The basic helix-loop-helix PER-ARNT-SIM (bHLH-PAS) domain-containing transcription factor CLOCK:BMAL1 forms the positive component of the core feedback loop. PER and CRY proteins interact with each other to form a large complex with the kinase CK1δ and enter the nucleus after a delay to bind directly to CLOCK:BMAL1 and inhibit its activity. What structural features of CRY1 and CRY2 might lead to differential functions in the circadian clock? Both cryptochromes are defined by a highly conserved photolyase homology region (PHR) domain and divergent C-terminal tails that are intrinsically disordered. However, repression also relies on the recruitment of CRY1 to the PAS domain core of CLOCK:BMAL1 via the CLOCK PAS-B domain, which docks into the evolutionarily conserved secondary pocket on the CRY1 PHR domain.

In addition to binding near the BMAL1 TAD-binding site at the CC helix of CRY1 and CRY2, the PER2 CBD also wraps around the distal side of the PHR domain to come into close contact with the serine loop (Nangle et al., 2014; Schmalen et al., 2014). To see if binding of the PER2 CBD truly alters the serine loop and secondary pocket of CRY1, we determined a crystal structure of the CRY1 PHR:PER2 CBD complex that eliminated this artifact. The overall conformation of the PER2 CBD in our structure is highly similar to the previously solved structure (0.76 Å Cɑ RMSD over PER2 residues 1136–1207). However, we now see that the serine loop maintains most of its flexibility in the PER2-bound state. Comparing the secondary binding pocket of the apo CRY1 PHR domain structure to our CRY1 PHR:PER2 CBD structure, we observed that PER2 CBD induces a modest structuring at the C-terminal end of the loop (residues 44–47). This reorganization is stabilized by an interaction between S45 on CRY1 and the backbone of Q1135 on the PER2 CBD. To determine if addition of the PER2 CBD alters binding between the CRY1 PHR domain and CLOCK:BMAL1, we utilized BLI binding assays using preformed CRY:PER2 CBD complexes with the immobilized PAS domain core and found that the CRY1:PER2 CBD complex binds with a ~ 3 fold reduction in affinity. Therefore, PER2 modestly weakens interaction of the CRY1 PHR domain with the CLOCK:BMAL1 PAS core, suggesting that this modest ordering of the CRY1 serine loop makes docking of the CLOCK PAS-B into the secondary pocket less favorable. Therefore, the addition of PER2 CBD causes the serine loops of CRY1 and CRY2 to take on a largely similar conformation, with the loop in CRY1 becoming more structured and the loop in CRY2 becoming less structured. Our data suggest that the differential effect of the PER2 CBD on CRY PHR binding to CLOCK:BMAL1 allows it to serve as a molecular equalizer—PER2 compensates for poorer binding by CRY2 by modestly enhancing its affinity for the transcription factor, while at the same time reducing CRY1 binding to bring the overall affinities of the two cryptochromes for the PAS domain core of CLOCK:BMAL1 to similar levels.

> MGVNAVHWFRKGLRLHDNPALKECIQGADTIRCVYILDPWFAGSSNVGINRWRFLLQCLEDLDANLRKLNSRLFVIRGQPADVFPRLFKEWNITKLSIEYDSEPFGKERDAAIKKLATEAGVEVIVRISHTLYDLDKIIELNGGQPPLTYKRFQTLVSKMEPLEMPADTITSDVIGKCMTPLSDDHDEKYGVPSLEELGFDTDGLSSAVWPGGETEALTRLERHLERKAWVANFERPRMNANSLLASPTGLSPYLRFGCLSCRLFYFKLTDLYKKVKKNSSPPLSLYGQLLWREFFYTAATNNPRFDKMEGNPICVQIPWDKNPEALAKWAEGRTGFPWIDAIMTQLRQEGWIHHLARHAVACFLTRGDLWISWEEGMKVFEELLLDADWSINAGSWMWLSCSSFFQQFFHCYCPVGFGRRTDPNGDYIRRYLPVLRGFPAKYIYDPWNAPEGIQKVAKCLIGVNYPKPMVNHAEASRLNIERMKQIYQQL;> GAMDPEFSSDTSHTSKYFGSIDSSENNHKAKMNTGMEESEHFIKCVLQDPIWLLMADADSSVMMTYQLPSRNLEAVLKEDREKLKLLQKLQPRFTESQKQELREVHQWMQTGGLPAAIDVAECVYCES Kinesin-8s are dual-activity motor proteins that can move processively on microtubules and depolymerize microtubule plus-ends, but their mechanism of combining these distinct activities remains unclear. The pathogenic yeast Candida albicans expresses a single kinesin-8 homolog, dubbed CaKip3, whose motor domain shares 60% sequence identity with that of S. cerevisiae Kip3. To understand the mechanistic basis for the dual-functionality of kinesin-8, we obtained seven cryo-EM structures of Candida albicans Kip3 bound to either the microtubule lattice or curved microtubule end mimics, and a microtubule-unbound CaKip3 X-ray structure. Our findings implicate loop-2 as a tubulin protofilament shape sensor that regulates conformational changes in the kinesin-8 motor domain, which can either induce curvature of protofilaments at the microtubule end, leading to microtubule depolymerization, or enable forward displacement of the neck linker for processive motility if the motor domain is bound to protofilaments in the microtubule lattice.

To visualize the microtubule-unbound ADP state of CaKip3, we determined a 2.0 Å X-ray crystal structure of a construct containing the motor domain and a slightly truncated neck-linker (CaKip3-MDN, residues 1–436). The CaKip3-MDN-ADP crystal structure has a partially open nucleotide pocket and an undocked neck-linker. The Switch I region (loop-9) is well-defined but angled away from ADP, while the Switch II region (loop-11) that coordinates microtubule sensing and nucleotide binding is mostly disordered. The electron density from the CaKip3-MDN-ADP crystal allowed us to model residues Phe116 to Ala131 of loop-2, which includes a proline-rich region and a ~10-residue helical sequence that is shared by some kinesin-8s.

>[2x]MASYPNSLGSPATVTSTSVPTAKQSSISVAVRVRPFTEAESNRLVKIDNDDVFLGDGCLTSDNNNNNNNSNSNGNGNGNGSSAANSSGASTSRRAIFNTLGGLRKIINVVDDRMLIFDPPETNPLTKMQRNAFPNSFKGSRIREHRFVFDRLFDEDCTQDQVYRNTTQPLLDSVLDGYNATVFAYGATGCGKTHTISGTPEDPGVIFLTMKELYNRIEELKDTKIIDISLSYLEIYNETIRDLLNPMTQCKNLVIREDANNKISVSNLSRHRPNSVEEVMQLILEGNKNRTCSPTEANATSSRSHAVLQINVIQKDRTGDITEEHTFATLSIIDLAGSERAAATKNRGARLNEGANINKSLLALGNCINALCDPRRRNHVPYRDSKLTRLLKFSLGGNCKTVMIVCVSPSSQHYDETLNTLKYADRAKEIKTKLIRNLEHHHHHH>[2x]MAREVKLTKAGYERLM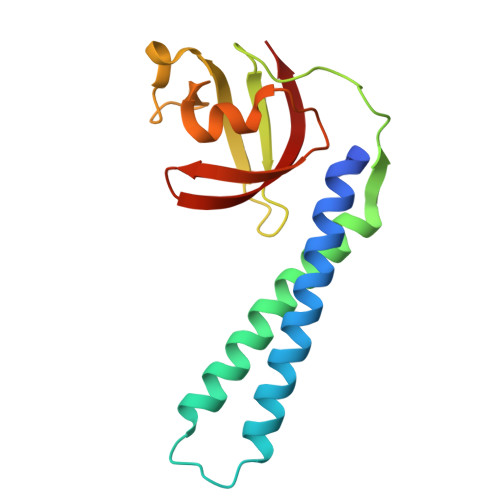QQLERERERLQEATKILQELMESSDDYDDSGLEAAKQEKARIEARIDSLEDILSRAVILEEGSGEVIGLGSVVELEDPLSGERLSVQVVSPAEANVLDTPMKISDASPMGKALLGHRVGDVLSLDTPKGKREFRVVAIHG> MKKITSVCALLSLICSFNA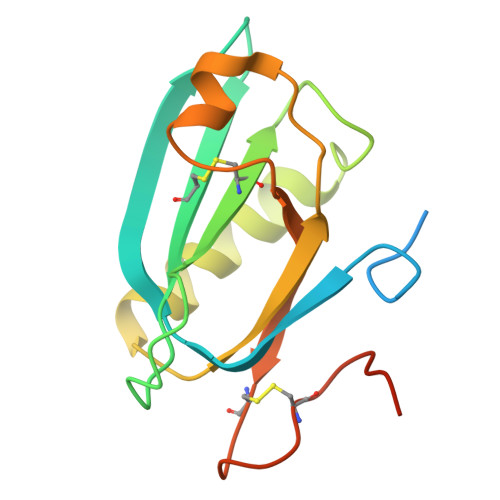SAEWTGDYENIGYFSHEVISEFHVGQIDGGAYFCIKAVKADGSRSTPLIACSVSNESVWAPSFKVLLEQARYFYVTEQSVRIYYDHNVWTNQPFVNTFSTNALVGLSSCSAATDCFGPGKPKSKSKRDVEQ> ADTVTLPFANGERPLVMYPGKRPLIGLTARPPQLETPFSVFDEGLITPNDAFFVRYHLAGIPLEIDPDAF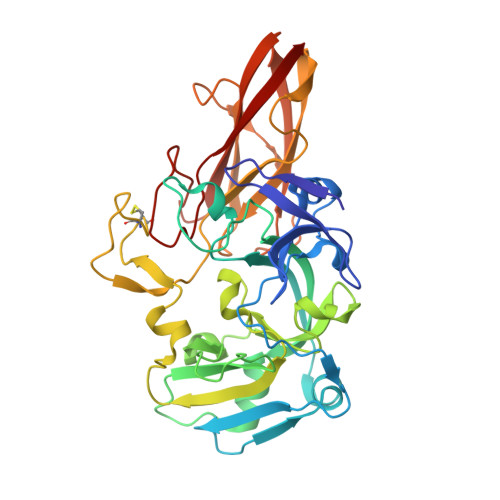RLEIKGKVGTPLSLSLQDLKNDFPASEVVAVNQCSGNSRGFVEPRVGGGQLANGAMGNARWRGVPLKAVLEKAGVQAGAKQVTFGGLDGPVIPETPDFVKALSIDHATDGEVMLAYSMNGADLPWLNGYPLRLVVPGYYGTYWVKHLNEITVIDKEFDGFWMKTAFRIPDNACACTEPGKAPTATIPINRFDVRSFITNVENGASVKAGEVPLRGIAFDGGYGITQVSVSADAGKSWTNATLDPGLGKYSFRGWKAVLPLTKGDHVLMCRATNARGETQPMQATWNPAGYMRNVVEATRVIAA>[4x]MVANPEHYIKHPLQNRWALWFFKND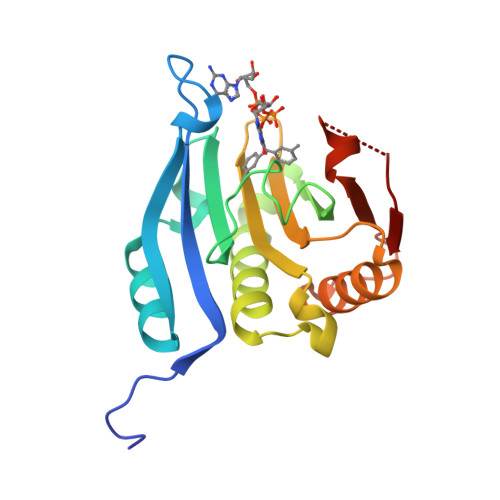KSKTWQANLRLISKFDTVEDFWALYNHIQLSSNLMPGCDYSLFKDGIEPMWEDEKNKRGGRWLITLNKQQRRSDLDRFWLETLLCLIGESFDDYSDDVCGAVVNVRAKGDKIAIWTTECENRDAVTHIGRVYKERLGLPPKIVIGYQSHADTATKSGSTTKNRFVV>MRGSHHHHHHGMASELALMDTTFQAAIDTGKINGAVVCATDAQGHFVYNKATGERTLLSGEKQPQQLDDVLYLASATKLITTIAALQCVEDGLLSLDGDLSSIAPELAAKYVLTGFTDDESPLDDPPARPITLKMLLTHSSGTSYHFLDPSIAKWRAQYANPENEKPRLVEEMFTYPLSFQPGTGWMYGPGLDWAGRVVERVTGGTLMEFMQKRIFDPLGITDSQFYPVTREDLRARLVDLNPSDPGALGSAVIGGGGEMNLRGRGAFGGHGLF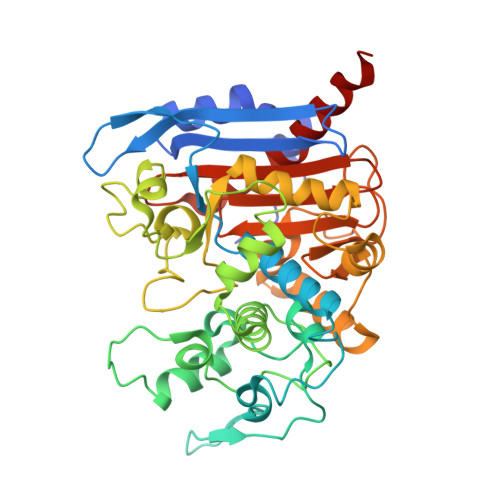LTGLDFVKILRSLLANDGMLLKPAAVDNMFQQHLGPEAAASHRAALASPLGPFFRVGTDPETKVGYGLGGLLTLEDVDGWYGERTLTWGGGLTLTWFIDRKNNLCGVGAIQAVLPVDGDLMADLKQTFRHDIYRKYSAWKGQQ[2x]3-[(3S)-oxolan-3-yl]-1-(pyrrolidin-1-yl)propan-1-one | C11 H19 N O2 | 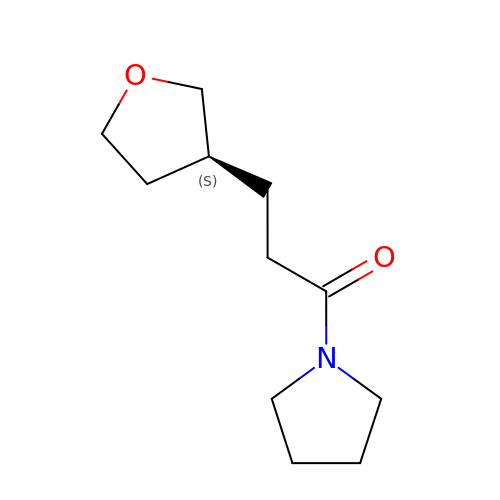QMNDAUGCAGNHLO-JTQLQIEISA-N>MMRIGELGKKADCLVQTVRFYESEGLLPEPARSEGNFRLYDEVHLQRLLFIRRCRAKDMTLDEIRQLLNLRDRPELGCGEVNALVDAHIAQVRTKMKELRALE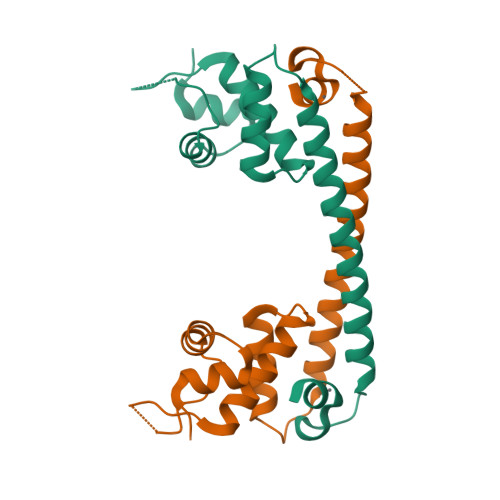RELMDLRRSCDSARTSRECGILNSLA[8x]> SMTDPEVFCFITKILCAHGGRMTLEELLGEISLPEAQLYELLKAAGPDRFVLLETGDQAGITRSVVATTRARVCRRKYCQRPCDSLHLCKLNLLGRCHYAQSQRNLCKYSHDVLSEQNFQVLKNHELSGLNQEE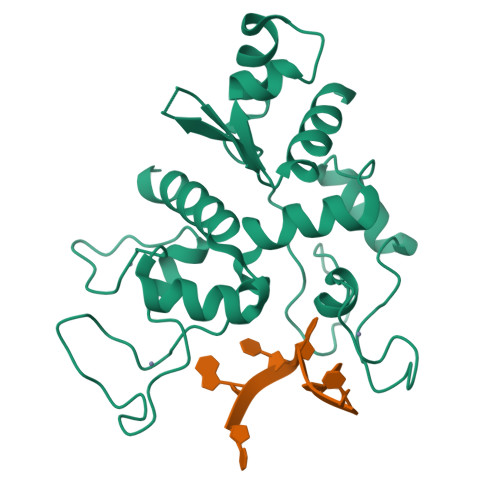LAVLLVQSDPFFMPEICKSYKGEGRKQICGQPQPCERLHICEHFTRGNCSYLNCLRSHNLMDRKVLAIMREHGLSSDVVQNIQDICNNKHTRRN> HHHHHHFNLPPGNYKKPKLLYCSNGGHFLRINPNGTVDGTRDRSDQHIQLQLSAESVGEVYIKSTETGQYLAMDTDGLLYGSQTPN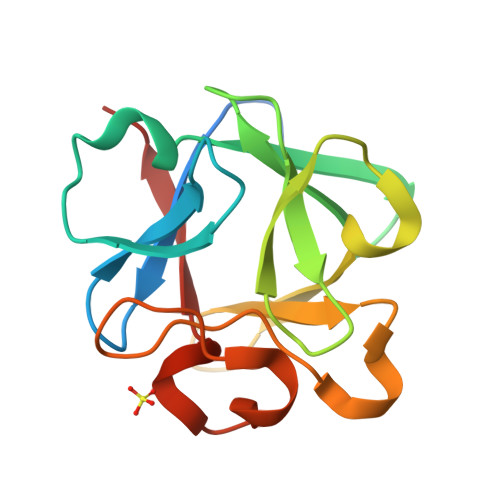EECLFLERLEENGYNTYISKKHAEKNWFVGLKKNGSCKRGPRTHYGQKAILFLPLPVSSD The human RAD52 protein, which forms an oligomeric ring structure, is involved in DNA double‐strand break repair. The N‐terminal half of RAD52 is primarily responsible for self‐oligomerisation and DNA binding.

However, only low‐resolution structures have been reported for the full‐length protein, and thus the structural role of the C‐terminal half in self‐oligomerisation has remained elusive. In this study, we determined the solution structure of the human RAD52 protein by cryo‐electron microscopy (cryo‐EM), at an average resolution of 3.5 Å. The structure revealed an undecameric ring that is nearly identical to the crystal structures of the N‐terminal half. The cryo‐EM map for the C‐terminal half was poorly defined, indicating that the region is intrinsically disordered. The present cryo‐EM structure provides important insights into the mechanistic roles played by the N‐terminal and C‐terminal halves of RAD52 during DNA double‐strand break repair.

>GSHMSGTEEAILGGRDSHPAAGGGSVLCFGQCQYTAEEYQAIQKALRQRLGPEYISSRMAGGGQKVCYIEGHRVINLANEMFGYNGWAHSITQQNVDFVDLNNGKFYVGVCAFVRVQLKDGSYHEDVGYGVSEGLKSKALSLEKARKEAVTDGLKRALRSFGNALGNCILDKDYLRSLNKLPRQLPLEVDLTKAKRQDLEPSVEEARYNSCRPNMALGHPQLQQVTSPSRPSHAVIPADQDCSSRSLSSSAVESEATHQRKLRQKQLQQQFRERMEKQQVRVSTPSAEKSEAAPPAPPVTHSTPVTVSEPLLEKDFLAGVTQELIKTLEDNSEKWAVTPDAGDGVVKPSSRADPAQTSDTLALNNQMVTQNRTPHSVCHQKPQAKSGSWDLQTYSADQRTTGNWESHRKSQDMKKRKYDPS[11x]>[2x]GPSAKNKEFFDALEEIAESAKNDETLRNELAKVLDDILKTDPSDPEAFRKIVAEHQEFWDEHDPSLMEFNEGRFFGKSRKQYLKSDDFLNSTDPTYNFQKLHQFAAEQRVKLGLEKSDTDTLVAILKNNPEECRAYIESKKPGLGNFSEGNVHGGSGGVLSDEAIKRIKEQARDLLLLKLINSSGNTQLLKDLRDAMSKPEAERAANALGFPTEGNGVLFLSREVVDALEERVEKLA

The effector RidL binds the Vps29 retromer subunit, blocks retrograde vesicle trafficking, and promotes intracellular bacterial replication. The 131-kDa Icm/Dot substrate RidL binds the retromer subunit Vps29 as well as PtdIns(3)P and impairs retrograde trafficking. Here, we show that the 29-kDa N-terminal domain of RidL (RidL2–281) adopts a “foot-like” fold comprising a protruding hydrophobic β-hairpin, which determines the interaction with the Vps29 retromer subunit and displaces the regulator TBC1D5 from the retromer. Thus, the hydrophobic β-hairpin of RidL is critical for binding of the L. pneumophila effector to the Vps29 retromer subunit and displacement of the regulator TBC1D5.

To test the possibility that deletion of the β-hairpin leads to global structural changes in RidL, we solved the structure of the N-terminal RidL fragment lacking the β-hairpin at 2.1 Å resolution. The N-terminal domain devoid of the β-hairpin crystallized in space group P212121 with two polypeptide chains (called molecule A and B) in the asymmetric unit. These molecules exhibited a root mean square deviation (RMSD) of 0.756 Å over 205 residues among each other, and mainly differ at the F-loop, which was partially undefined due to the high flexibility in molecule A. Superpositions of the Δβ-hairpin mutant with the wild-type RidL domain over the same 205 residues resulted in RMSD of 0.872 Å and 0.962 Å for molecules A and B, respectively (Fig. 1f features the superimposition of molecule B). Thus, the N-terminal RidL fragment lacking the β-hairpin adopts an overall structure that is very similar to the parental fragment. Interestingly, the fragment lacking the β-hairpin no longer co-localized with the retromer and was found throughout the cell. As expected, the Δβ-hairpin mutant did not reveal any detectable binding to Vps29. The SEC analysis of RidL-ΔF-loop or RidL-Δβ-hairpin deletion proteins did not reveal any changes in the elution behavior compared to RidL, indicating that the mutants are correctly folded. In contrast, the addition of RidL10–258-Δβ-hairpin or buffer only did not result in the elution of the retromer. Thus, RidL10–258 displaces the retromer from TBC1D5 in a β-hairpin-dependent manner.>MKCLVVGHVVRDIVKKGNKVLERLGGGAYYSALALSRFCDVEILTSFSNLPEEWIKELE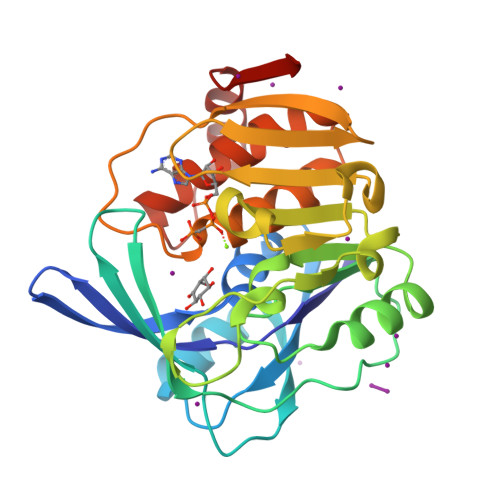SMAKLQVVPSETTTTYELTYLDGNRRRLKLLERASPIEELPDGEYDVLLMNPVAREVPPALVTSALKKFPFVAVDIQGFIRSSSPGEIQYQPIDGSFLKGVKILHADLGEYQYLQGFSPEFVDVLLLSNGPEPGKAFLHGREYTFEPVHVGVDESTGAGDVFLGAFTGFYSQCPFVQALKRAAAFTALFLKNRSVDFSMDDVNELAMKVEVKRV[2x]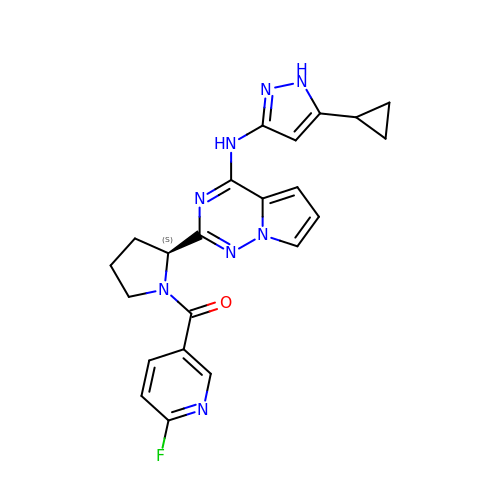N-(5-cyclopropyl-1H-pyrazol-3-yl)-2-{(2S)-1-[(6-fluoropyridin-3-yl)carbonyl]pyrrolidin-2-yl}pyrrolo[2,1-f][1,2,4]triazin-4-amine | C22 H21 F N8 O | XXGADWBTSMHVDF-INIZCTEOSA-N> MPNPDNTEAHVAGEVEIENSAIALSGIVSVANNADNRLEVFGVSTDSAVWHNWQTAPLPNSSWAGWNKFNGVVTSKPAVHRNSDGRLEVFVRGTDNALWHNWQTAADTNTWSSWQPLYGGITSNPEVCLNSDGRLEVFVR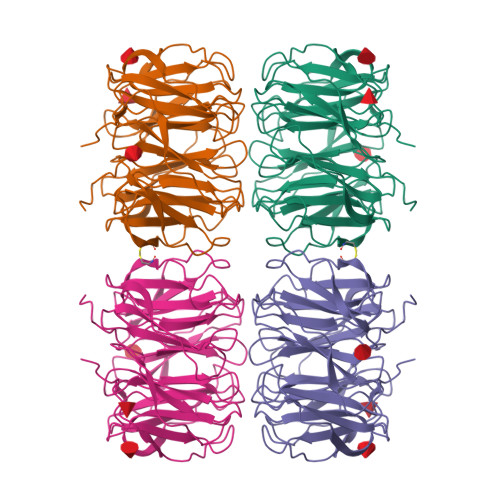GSDNALWHIWQTAAHTNSWSNWKSLGGTLTSNPAAHLNADGRIEVFARGADNALWHIWQTAAHTDQWSNWQSLKSVITSDPVVINNCDGRLEVFARGADSTLRHISQIGSDSVSWSNWQCLDGVITSAPAAVKNISGQLEVFARGADNTLWRTWQTSHNGPWSNWSSFTGIIASAPTVAKNSDGRIEVFVLGLDKALWHLWQTTSSTTSSWTTWALIGGITLIDASVILEHHHHHHWRSGC> MGKYLLPTAAAGLLLLAAQPAMDFTIQDIRVEGLQRTEPSTVFNYLPVKVGDTYNDTHGSAIIKSLYATGFFDDVRVETADGQLLLTVIERPTIGSLNITGAKMLQNDAIKKNLESFGLAQSQYFNQATLNQAVAGLKEEY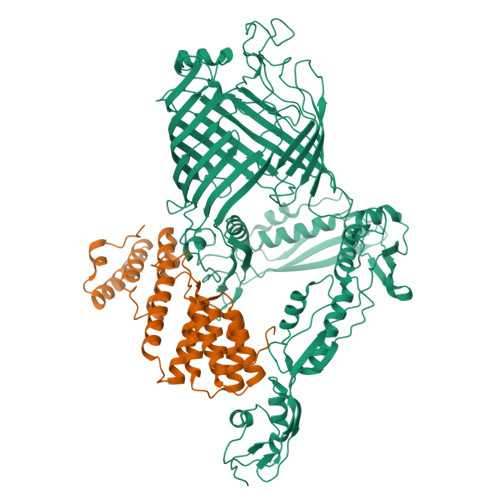LGRGKLNIQITPKVTKLARNRVDIDITIDEGKSAKITDIEFEGNQVYSDRKLMRQMSLTEGGIWTWLTRSDRFDRQKFAQDMEKVTDFYQNNGYFDFRILDTDIQTNEDKTRQTIKITVHEGGRFRWGKVSIEGDTNEVPKAELEKLLTMKPGKWYERQQMTAVLGEIQNRMGSAGYAYSEISVQPLPNAGTKTVDFVLHIEPGRKIYVNEIHITGNNKTRDEVVRRELRQMESAPYDTSKLQRSKERVELLGYFDNVQFDAVPLAGTPDKVDLNMSLTERSTGSLDLSAGWVQDTGLVMSAGVSQDNLFGTGKSAALRASRSKTTLNGSLSFTDPYFTADGVSLGYDIYGKAFDPRKASTSVKQYKTTTAGGGVRMGIPVTEYDRVNFGLAAEHLTVNTYNKAPKRYADFIRKYGKTDGADGSFKGLLYKGTVGWGRNKTDSASWPTRGYLTGVNAEIALPGSKLQYYSATHNQTWFFPLSKTFTLMLGGEVGIAGGYGRTKEIPFFENFYGGGLGSVRGYESGTLGPKVYDEYGEKISYGGNKKANVSAELLFPMPGAKDARTVRLSLFADAGSVWDGRTYTAAENGNNKSVYSENAHKSTFTNELRYSAGGAVTWLSPLGPMKFSYAYPLKKKPEDEIQRFQFQLGTTF;> MQLRKLLLPGLLSVTLLSGCAMGATQGTADKDAQITQDWSVEKLYAEAQDELNSSNYTRAVKLYEILESRFPTSRHARQSQLDTAYAYYKDDEKDKALAAIERFRRLHPQHPNMDYALYLRGLVLFNEDQSFLNKLASQDWSDRDPKANREAYQAFAELVQRFPNSKYAADATARMVKLVDALGGNEMSVARYYMKRGAYIAAANRAKKIIGSYQNTRYVEESLAILELAYKKLDKPQLAADTRRVLETNFPKSPFLTHAWQPDDMPWWRYWH2-[1-METHYLHEXYL]-4,6-DINITROPHENOL | C13 H18 N2 O5 | 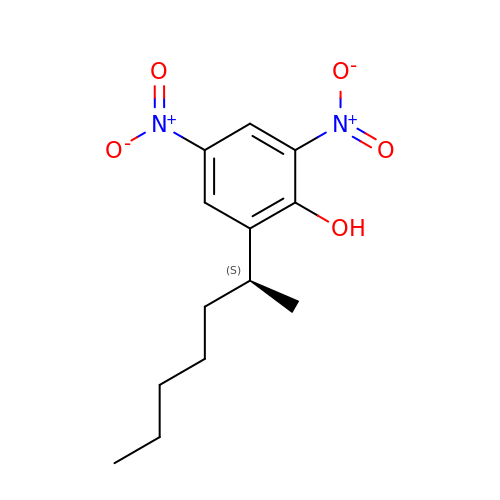RROCMCBQTUYDSD-UHFFFAOYSA-N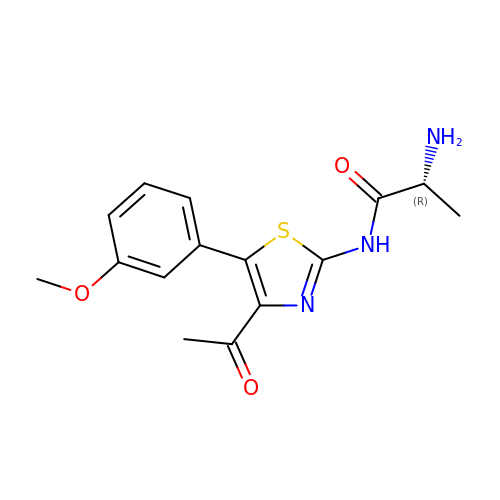(2~{R})-2-azanyl-~{N}-[4-ethanoyl-5-(3-methoxyphenyl)-1,3-thiazol-2-yl]propanamide | C15 H17 N3 O3 S | RXAAAHIWJRPSEA-MRVPVSSYSA-N>[2x]ADLLSKFDPLIAEREALLATGVRDPYAIVMDKVLSPTEAMINGRKTILLGTYNYMGMTFDPDVIAAGKQALDEFGSGTTGSRVLNGTYQGHKACEDALKEFYGTEHAIVFSTGYQANLGMISTLAGKGDYIILDADSHASIYDGCWLGDAEIVRFRHNSVEDLDKRLGRLPAEAGKLVVLEGVYSMMGDIAPLQEMVAVSKKHGAMILVD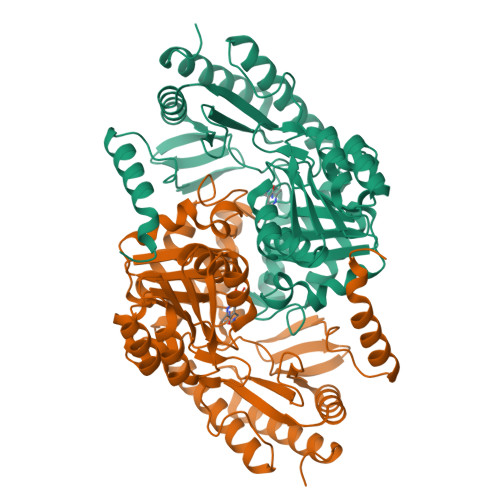EAHGMGFFGEHGRGVFEEAGVEADVDFVVGTFSKSVGTVGGFCVSNHPKFEVLRLVCRPYVFTASLPPSVVATAATSIRKLMHAGDKRAHLWKNSRRLHQGLRDMGYKLGTETAQSAIIAVILTDMAQAVALWQGLLEAGLYVNTARPPATPAGMFLLRCSLCAEHSDEQVEQILGMFESAGRATGVIPKLAAALEHHHHHH>MKEAFKEALARFASGVTVVAARLGEEERGMTATAFMSLSLEPPLVALAVSERAKLLPVLEGAGAFTVSLLREGQEAVSEHFAGRPKEGIALEEGRVK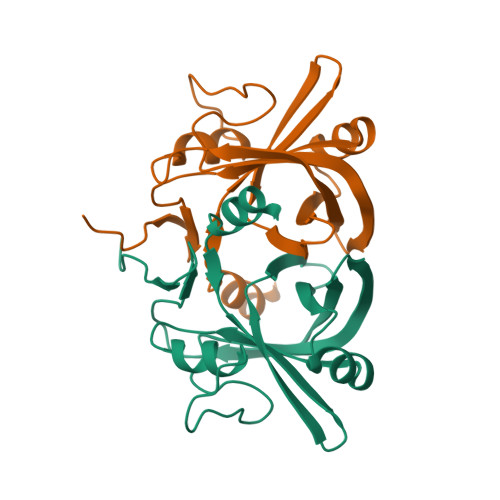GALAVLRCRLHALYPGGDHRIVVGLVEEVELGEGGPPLVYFQRGYRRLVWPS[2x]MACBECIN | C30 H42 N2 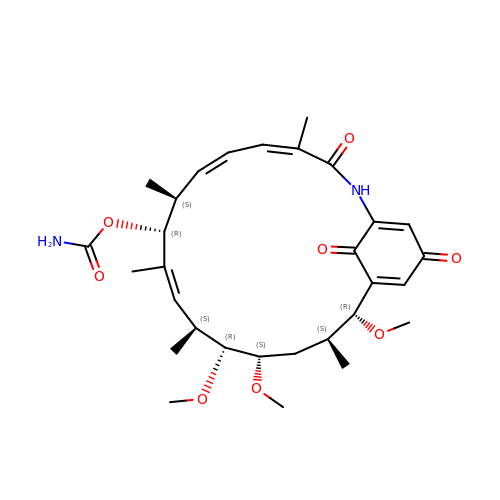O8 | PLTGBUPHJAKFMA-CISVGLRTSA-N>GAHMAGRSMQAARCPTDELSLSNCAVVSEKDYQSGQHVIVRTSPNHKYIFTLRTHPSVVPGSVAFSLPQRKWAGLSIGQEIEVALYSFDKAKQCIGTMTIEIDFLQKKNIDSNPYDTD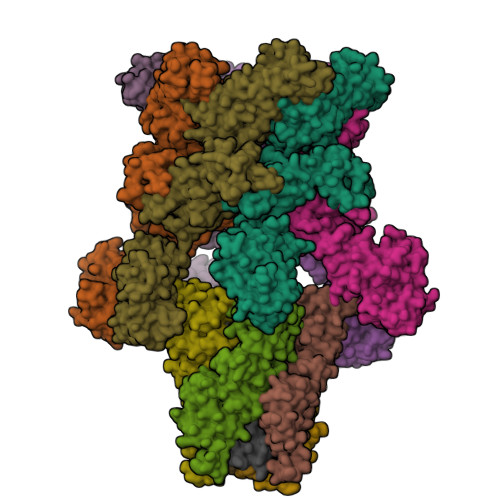KMAAEFIQQFNNQAFSVGQQLVFSFNDKLFGLLVKDIEAMDPSILKGEPASGKRQKIEVGLVVGNSQVAFEKAENSSLNLIGKAKTKENRQSIINPDWNFEKMGIGGLDKEFSDIFRRAFASRVFPPEIVEQMGCKHVKGILLYGPPGCGKTLLARQIGKMLNAREPKVVNGPEILNKYVGESEANIRKLFADAEEEQRRLGANSGLHIIIFDEIDAICKQRGSMAGSTGVHDTVVNQLLSKIDGVEQLNNILVIGMTNRPDLIDEALLRPGRLEVKMEIGLPDEKGRLQILHIHTARMRGHQLLSADVDIKELAVETKNFSGAELEGLVRAAQSTAMNRHIKASTKVEVDMEKAESLQVTRGDFLASLENDIKPAFGTNQEDYASYIMNGIIKWGDPVTRVLDDGELLVQQTKNSDRTPLVSVLLEGPPHSGKTALAAKIAEESNFPFIKICSPDKMIGFSETAKCQAMKKIFDDAYKSQLSCVVVDDIERLLDYVPIGPRFSNLVLQALLVLLKKAPPQGRKLLIIGTTSRKDVLQEMEMLNAFSTTIHVPNIATGEQLLEALELLGNFKDKERTTIAQQVKGKKVWIGIKKLLMLIEMSLQMDPEYRVRKFLALLREEGASPLDFD[6x];>[4x]GSMDTSGKQAEAMALLAEAERKVKNSQSFFSGLFGGSSKIEEACEIYARAANMFKMAKNWSAAGNAFCQAAQLHLQLQSKHDAATCFVDAGNAFKKADPQEAINCLMRAIEIYTDMGRFTIAAKHHISIAEIYETELVDVEKAIAHYEQSADYYKGEESNSSANKCLLKVAGYAAQLEQYQKAIDIYEQVGTSAMDSPLLKYSAKDYFFKAALCHFCIDMLNAKLAVQKYEELFPAFSDSRECKLMKKLLEAHEEQNVDSYTESVKEYDSISRLDQWLTTMLLRIKKTIQGDEEDLR;> GSNRRLQQTQAQVDEVVDIMRVNVDKVLERDQKLSELDDRADALQAGASQFETSAAKLKRKYW;> MALSEIETRHSEIIKLENSIRELHDMFMDMAMLVESQGEMIDRIEYNVEHAVDYVERAVSDTKKAVK;> RADQLADESLESTRRMLQLVEESKDAGIRTLVMLDEQGEQLDRVEEGMNHINQDMKEAEKNLKDLGKFCGLCVCPCNKLKSSDAYKKAWGNNQDGVVASQPARVVDEREQMAISGGFIRRVTNDARENEMDENLEQVSGIIGNLRHMALDMGNEIDTQNRQIDRIMEKADSNKTRIDEANQRATKMLG>MGHHHHHHHHMATLTAKNLAKAYKGRRVVEDVSLTVNSGEIVGLLGPNGAGKTTTFYMVVGIVPRDAGNIIIDDDDISLLPLHARARRGIGYLPQEASIFRRLSVYDNLMAVLQIRDDLSAEQREDRANELMEEFHIEHLRDSMGQSLSGGERRRVEIARALAANPKFILLDEPFAGVDPISVIDIKRIIEHLRDSGLGVLITDHNVRETLAVCERAYIVSQGHLIAHGTPTEILQDEHVKRVYLGEDFRL[2x];> MIIIRYLVRETLKSQLAILFILLLIFFCQKLVRILGAAVDGDIPANLVLSLLGLGVPEMAQLILPLSLFLGLLMTLGKLYTESEITVMHACGLSKAVLVKAAMILAVFTAIVAAVNVMWAGPWSSRHQDEVLAEAKANPGMAALAQGQFQQATNGSSVLFIESVDGSDFKDVFLAQIRPKGNARPSVVVADSGHLTQLRDGSQVVTLNQGTRFEGTALLRDFRITDFQDYQAIIGHQAVALDPNDTDQMDMRTLWNTDTDRARAELNWRITLVFTVFMMALMVVPLSVVNPRQGRVLSMLPAMLLYLLFFLIQTSLKSNGGKGKLDPTLWMWTVNLIYLALAIVLNLWDTVPVRRLRASFSRKGAV;> MQPF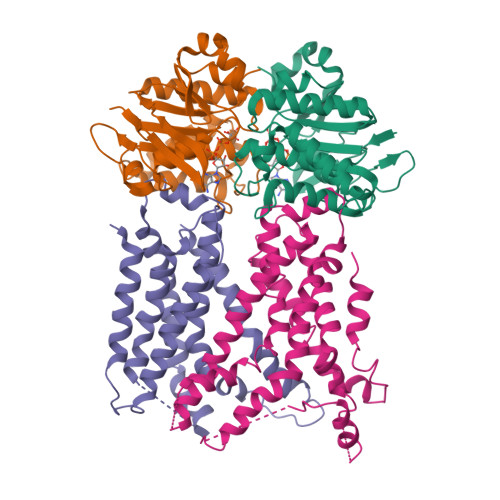GVLDRYIGKTIFTTIMMTLFMLVSLSGIIKFVDQLKKAGQGSYDALGAGMYTLLSVPKDVQIFFPMAALLGALLGLGMLAQRSELVVMQASGFTRMQVALSVMKTAIPLVLLTMAIGEWVAPQGEQMARNYRAQAMYGGSLLSTQQGLWAKDGNNFVYIERVKGDEELGGISIYAFNENRRLQSVRYAATAKFDPEHKVWRLSQVDESDLTNPKQITGSQTVSGTWKTNLTPDKLGVVALDPDALSISGLHNYVKYLKSSGQDAGRYQLNMWSKIFQPLSVAVMMLMALSFIFGPLRSVPMGVRVVTGISFGFVFYVLDQIFGPLTLVYGIPPIIGALLPSASFFLISLWLLMRKS>[2x]MGHHHHHHGSGSNRLDGKVAIITGGTLGIGLAIATKFVEEGAKVMITGRHSDVGEKAAKSVGTPDQIQFFQHDSSDEDGWTKLFDATEKAFGPVSTLVNNAGIAVNKSVEETETAEWRKLLAVNLDGVFFGTRLGIQRMKNKGLGASIINMSSIEGFVGDPSLGAYNASKGAVRIMSKSAALDCALKDYDVRVNTVHPGYIKTPLVDDLPGAEEAM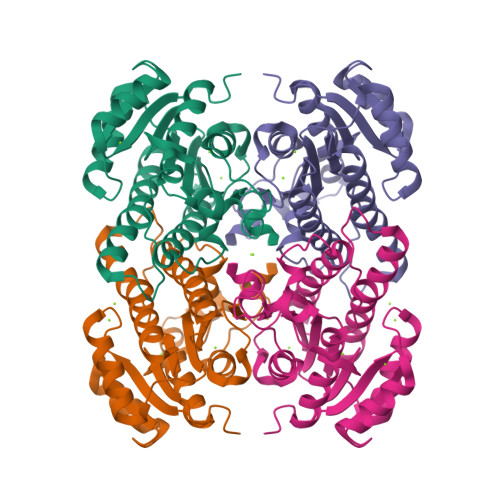SQRTKTPMGHIGEPNDIAYICVYLASNESKFATGSEFVVDGGYTAQ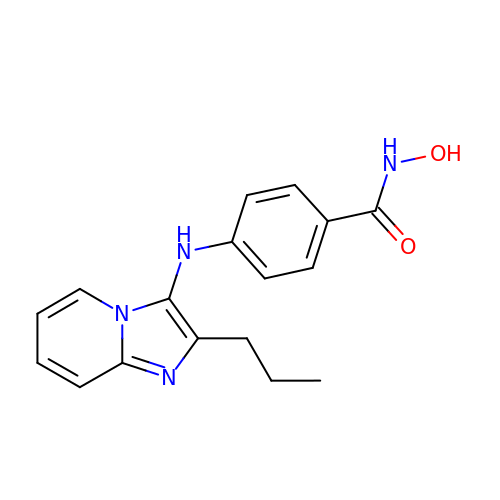N-hydroxy-4-[(2-propylimidazo[1,2-a]pyridin-3-yl)amino]benzamide | C17 H18 N4 O2 | RDGVRQVQYOOAEK-UHFFFAOYSA-N(2S)-2-NITROBUTANE | C4 H9 N O2 | 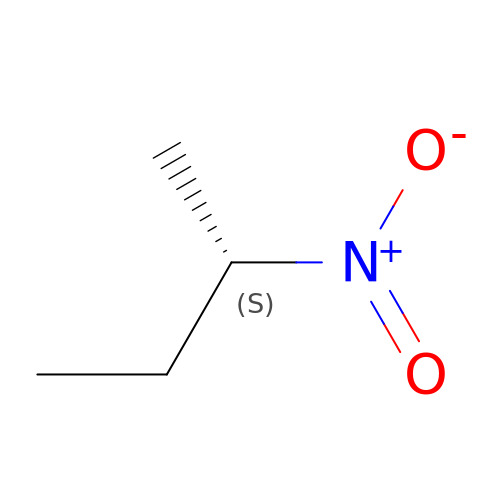SUGZATOHBPXTDV-BYPYZUCNSA-N> GPGSEF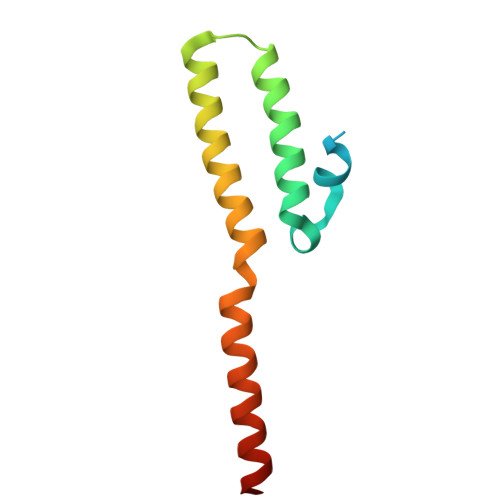MEDHPVREEEDGEEDEGALAKSPLQLTTDDVYDISYVVGRELMALGSDPRVTRLQFKIVRVMEMLETLVNEGSLAVEELRMERDNLKQEVEGLRKAG>GDHGPEFNGVMVVKAAEAEELPDDLMNFKGTWEVSADGSSGRFFSKGATDSYVFHLIPAKDVKKPGWREHNEVKDSYIKIDKQSIAARYKTSTTAPYSVAFKVNTKSLIKDHDYKITFEQGQIASGITVDYRIGSAFNKTTDDSFKISDESKYASNVKIEGEEQGFKQREQGDKTISFRTLKEGPMSLVLLSKVEKKPQGDLDVEFKNLKIIDVTNPSQLDKGVAYVGNKNVQLTLKSDDGRTNFEGDEISLFNSRGELLQTVTVTKDQQNPI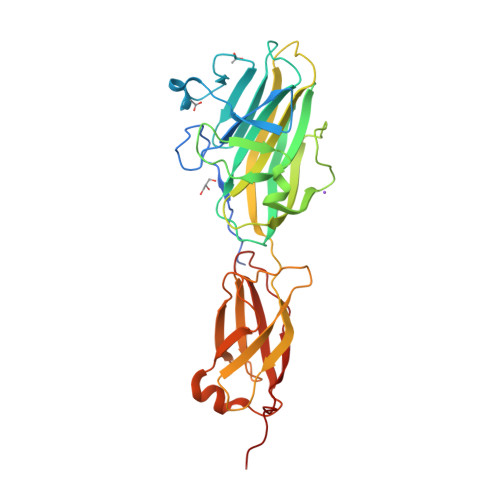SITLSEDQAKSLKNKEKLKVSIKQKQSKKTSKDFFFEVGIDPKVEAK[2x]>GHMASMNRTLT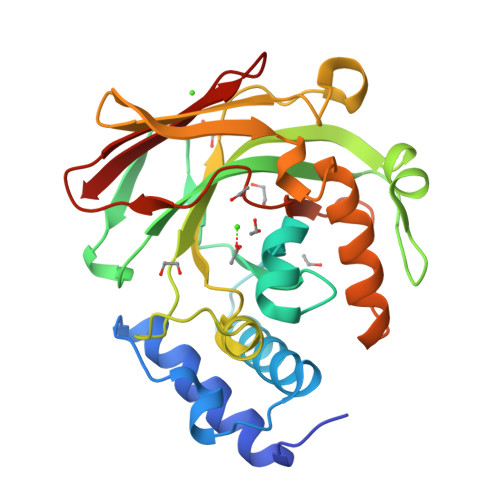REQVLALAEHIENAELNVHDIGKVTNDFPEMTFADAYDVQWEIRRRKEARGNKIVGLKMGLTSWAKMAQMGVETPIYGFLADYFSVPDGGVVDCSKLIHPKIEAEISVVTKAPLHGPGCHLGDVIAAIDYVIPTVEVIDSRYENFKFDPISVVADNASSTRFITGGRMASLEEVDLRTLGVVMEKNGEVVELGAGAAVLGHPLSSVAMLANLLAERGEHIPAGTFIMTGGITAAVPVAPGDNITVRYQGLGSVSARFI[2x]>MTTQPQLKENLTQWAYLALNSELNIADGHARQALSPGQQKIVNELPVLWAESEQRPVQQIESEAHQAYFTLLGQHGYPAEPGRVLSCYSSSVSMEILARSLSASVDRVALVHPTFDNIADLLRGNGLDLVPVEEDALHGADLSAELLSSVGCVFVTTPNNPTGRVLAEERLRRLAEQCAEHGTVLALDTSFRGFDAAAHYDHYAVLQEAGCRWVVIEDTGKLWPTLDLKAGLLVFSEDIGLPVEKIYSDILLGVSPLILALIREFSRDAADGGLADLHAFILHNRSV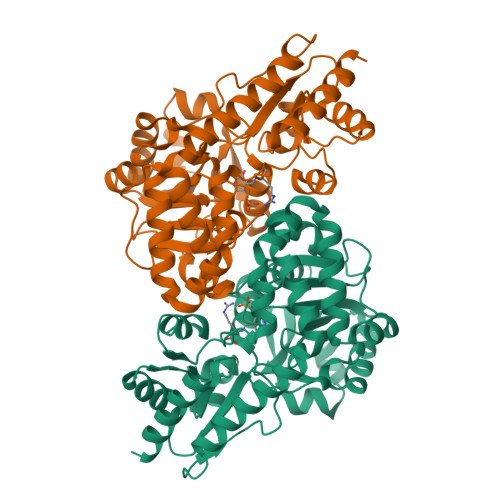VRRALAGVEGVSFPDPESRSSVERVAFAGRTGTEVWEELQRHHVFALPCRQFHWAEPSDGDHMVRIALSRSTEPLEKSVQVLRTVLETR[8x]>TSLAVTEPEVNDEFTGDKEAYMASVLARYRKTLVERTKNHLGYPYNLDFDYGALGQLQHFSINNLGDPFIESNYGVHSRPFEVGVLDWFARLWEIERDDYWGYITNCGTEGNLHGILVGREMFPDGILYASRESHYSVFKAARMYRMECEKVDTLMSGEIDCDDLRKKLLANKDKPAILNVNIGTTVKGAVDDLDLVIKTLEECGFSHDRFYIHCDGALFGLMMPFVKRAPKVTFNKPIGSVSVSGHKFVGCPMPCGVQITRMEHIKVLSSNVEYLASRDATIMGSRNGHAPLFLWYTLNRKGYKGFQKEVQKCLRNAHYLKDRLREAGISAMLNELSSTVVFERPKDEEFVRRWQLACQGDIAHVVVMPSVTIEKLDNFLKDLVKHRLIWYEDGSQPPCLASEVGTNNCICPAHKAA[4x]

Ethylamine (EA), the precursor of theanine biosynthesis, is synthesized from alanine decarboxylation by alanine decarboxylase (AlaDC) in tea plants. In this study, we solved the X-ray crystal structures of AlaDC from Camellia sinensis (CsAlaDC) and SerDC from Arabidopsis thaliana (AtSerDC). CsAlaDC and AtSerDC are Group II PLP-dependent amino acid decarboxylases, which exhibit numerous structural features common to other amino acid decarboxylases. The overall structure of CsAlaDC or AtSerDC is homodimeric with two subunits exhibiting an asymmetrical arrangement.

Through optimization of crystallization conditions, we successfully determined the crystal structures of CsAlaDC, CsAlaDC-EA, and AtSerDC at resolutions of 2.50 Å, 2.60 Å, and 2.85 Å, respectively. The crystal structures of the CsAlaDC-EA complex and AtSerDC were obtained and further analyzed. Additionally, His308, Gly169, Thr170, Lys309, and Ser347*(‘*’ denotes the amino acids on adjacent subunits) establish a hydrogen bonding network with the phosphate group of PLP, consequently fortifying its attachment to the protein. Similarly, in the latter structure, the pyridine ring of PLP was sandwiched between the imidazole ring of His201 and the methyl group of Ala284. The N1 of PLP formed a salt bridge with Asp282, while the O3 formed hydrogen bonds with Thr252. The phosphate group of PLP established hydrogen bonding interactions with Lys314, His313, Gly174, Thr175, and Ser352*. The catalytic loop in AtSerDC, consisting of amino acid residues 328–341, is well-structured and exhibits clear electron density. The superposition of amino acid residues in the substrate binding pocket of CsAlaDC and AtSerDC revealed that all residues are identical, except for the substitution of Tyr at position 111 in AtSerDC with Phe at position 106 in CsAlaDC. The results revealed that AtSerDCY111F acquired alanine decarboxylase activity, whereas CsAlaDCF106Y completely lost its alanine decarboxylase activity. Moreover, compared with AtSerDC, the serine decarboxylase activity of AtSerDCY111F was about 30% of AtSerDC; AtSerDCY111I retained lower than 5% of serine decarboxylase activity of AtSerDC; while other mutations, including AtSerDCY111A, AtSerDCY111L, AtSerDCY111V, and AtSerDCY111W abolished the serine decarboxylase activity. These results suggested the Tyr111 of AtSerDC is also important for the selective binding of serine for AtSerDC.Fra a proteins are members of the pathogenesis-related 10 family and are required for the normal accumulation of flavonoids and the development of color in strawberry fruits. PR-10 proteins belong to the START superfamily. These proteins adopt a helix-grip fold with an internal cavity capable of binding hydrophobic ligands. The data presented here demonstrates that Fra a proteins bind natural flavonoids, providing for the first time mechanistic insight on the function of these proteins in the control of flavonoid biosynthesis.

In the case of Fra a 3, crystals were obtained only in the presence of catechin, a natural flavonoid present in strawberries. The crystallographic model contains five protein chains and six molecules of catechin. All of the molecules of Fra a 3 in the asymmetric unit showed additional density inside the cavity. This density could be easily interpreted as (+)-catechin. The catechin molecule inside of the Fra a 3 binding cavity is stabilized both by polar and hydrophobic interactions and shows the same conformation in the five copies within the asymmetric unit. The flavan nucleus is oriented with its long axis approximately parallel to the helix α3 and with the B ring pointing toward the bottom of the cavity. The catechin molecule adopts a linear disposition with its long axis approximately parallel to the axis of the long C-terminal α-helix of Fra a 3. It is stabilized by polar interactions with the side chains of Asp-28, Ser-63, His-70, Tyr-84, and Arg-139 and backbone atoms of residues Gln-37, Ala-38, and Gly-60, whereas the non-polar groups of catechin are surrounded by hydrophobic side chains including Ile-31, Val-39, Leu-59, and Leu-143. In the Fra a 3 structure, the loop L5 wraps around one end of the catechin molecule and approaches the C-terminal α-helix (α3) on the opposite side restricting the access to the cavity. At the same time, helix α3 of Fra a 3 shows a slight bend at its center toward loop L5, whereas loop L3 approaches loop L5 and the ligand. This closed conformation is stabilized by interactions with the catechin molecule.

>[5x]AMAGVFTYESEFTSVIPPPKLFKAFVLDADNLIPKIAPQAVKSAEIIEGDGGVGTIKKIHLGEGSEYSYVKHKIDGIDKDNFVYSYSIIEGDAIGDKIEKISYEIKLVASGGGSIIKSTSHYHTKGEVEIKEEHVKAGKERAAGLFKIIENHLLAHPEEYN>[6x]SDGGAQDCCLKYSQRKIPAKVVRSYR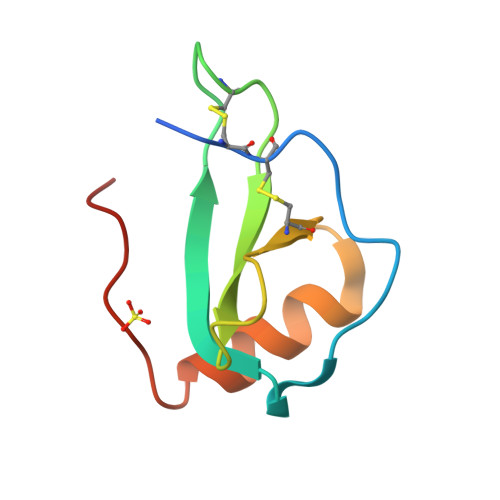KQEPSLGCSIPAILFLPRKRSQAELCADPKELWVQQLMQHLDKTPSPQKPAQG>MQPINTSNPDNTASYVKD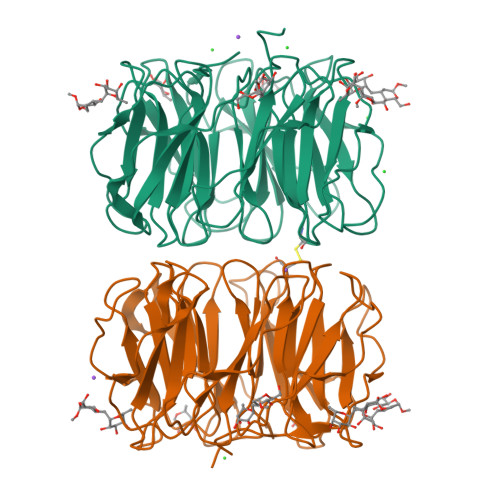EVEITSSTIALSEIVSVVNTSDGRLEVFGVGTDKAVWHNRQMAPHTGSPWSGWSSLKGQVTSKPVVYINTDGRLEVFARGTDNALWHIWQTATNAGWSNWQSLGGVITSNPAIYANTDGRLEVFARGADNALWHISQTTAHSGPWSSWASLNGVITSNPTVHINSDGRLEVFARGTDNALWHIWQTAPDSNLWSSWESLNGIITSDPVVIDTADGRLEVFARGADNALWHIWQTISHSGPWSGWQSLNGVITSAPAVAKNCDNRLEAFARGTDNALWHTWQTVSHSGPWSSWQSLNGVITSAPTAVRDADGRLEVFARGTDNALWLTWQTASSWSPWISLGGVLIDASAIK[2x]We have described functional and structural studies involving a toxin isolated from Bothrops moojeni venom, MjTX-II, and the inhibitor Varespladib. On the other hand, Lys49-PLA2-like myotoxins share the same general scaffold as Asp49-PLA2s, but display myotoxicity in the absence of catalysis. A hypothesis on the mechanism of myotoxicity induced by Lys49-PLA2-like toxins was recently presented, and involves several steps. It is proposed that initiation occurs by the binding of a fatty acid into the hydrophobic channel of the toxin, followed by allosteric activation and alignment of functional sites.

The crystal structure of the complex MjTX-II/Varespladib reveals the presence of inhibitor molecules in the hydrophobic channel of the toxin, interacting particularly with His48 and Lys49 residues. The structural importance of these residues was also observed by MD simulation, in which they were found to interact with the ligand during almost the whole time. Therefore, binding of Varespladib into the toxin’s hydrophobic channel is likely to prevent the membrane’s fatty acids binding and, consequently, precludes the structural alignment of the functional MDoS and MDiS regions, resulting in reduction of toxicity. Another structural feature observed was the particular dimeric assembly of MjTX-II/Varespladib when compared to other PLA2-like toxins. On the other hand, Varespladib maintains strong interactions with the same regions (Helix-I: Leu2, Leu5, Gly6 and Ile9 residues; MDiS: Leu122 and Phe126 residues; and residues His48 and Lys49), as observed in the crystal structure and MD simulations, occupying the hydrophobic channel internally. The interaction of Varespladib with residues of the hydrophobic channel forces MDiS to remain in contact with the toxin, favoring the distorted conformation. In the present work, MD simulation of the MjTX-II/Varespladib complex showed high stability and affinity of the inhibitor in the binding site on hydrophobic channel, which suggests that Varespladib prevents the interaction of fatty acids with the toxin by competitive inhibition, and also preserves the distorted structure of the toxin. In the present study, functional assays performed in mice and in cell culture demonstrated that Varespladib interacts with MjTX-II leading to a significant inhibition of its myotoxic and cytotoxic effects.

>[2x]SLFELGKMILQETGKNPAKSYGVYGCNCGVGGRGKPKDATDRCCYVHKCCYKKLTGCDPKKDRYSYSWKDKTIVCGENNSCLKELCECDKAVAICLRENLDTYNKKYRYNYLKPFCKKADPC>MGSSHHHHHHSSGENLYFQGVPTVQRGIIKMVLSGCAIIVRGQPRGGPPPERQINLSNIRAGNLARRAAKDTPDEPWAFPAREFLRKKLIGKEVCFTIENKTPQGREYGMIYLGKDTNGENIAESLVAEGLATRREGMRANNPEQNRLSECEEQAKAAKKGMWSEGNGSHTIRDLKYTIENPRHFVDSHHQKPVNAIIEHVRDGSVVRALLLPDYYLVTVMLSGIKCPTFRRETPEPFAAEAKFFTESRLLQRDVQIILESCHNQNILGTI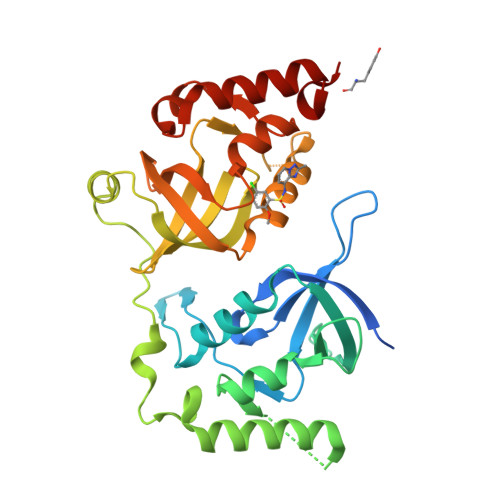LHPNGNITELLLKEGFARCVDWSIAVYTRGAEKLRAAERFAKERRLRIWRDYV[4x]> MASWSHPQFEKSGGGGGENLYFQGAVLALERHFEKVEEILKKYGYKRENLIKILLEIQEIYRYLPEDVINYVSTAMGIPPAKIYGVATFYAQFSLKPKGKYTIMVCDG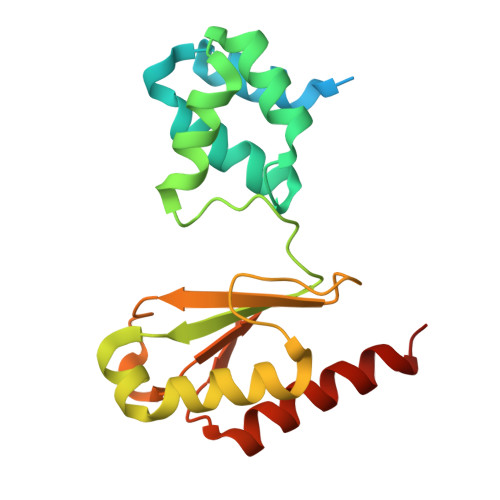TACHMAGSPEVLKAIEEETGLTPGNVTEDLMFSLDQVGCLGACALAPVMVINGEVYGNLTADKVKEILRKIKEKERESANV>GSNLEERLRACMQKLACGKLTGISDPVTVKTSGSRFGSWMTDPLAPEGDNRVWYMDGYHNNRFVREYKSMVDFMNTDNFTSHRLPHPWSGTGQVVYNGSIYFNKFQSHIIIRFDLKTETILKTRSLDYAGYNNMYHYAWGGHSDIDLMVDENGLWAVYATNQNAGNIVISKLDPVSLQILQTWNTSYPKRSAGEAFIICGTLYVTNGYSGGTKVHYAYQTNASTYEYIDIPFQNKYSHISMLDYNPKDRALYAWNNGHQTLYNVTLFHAAAHHHHHH[2x]

Olfactomedin-1 (Olfm1; also known as Noelin or Pancortin) is a highly-expressed secreted brain and retina protein and its four isoforms have different roles in nervous system development and function. Structural studies showed that the long Olfm1 isoform BMZ forms a disulfide-linked tetramer with a V-shaped architecture. The tips of the Olfm1 “V” each consist of two C-terminal β-propeller domains that enclose a calcium binding site. The highly conserved monomeric Olf domain has a five-bladed β-propeller fold with a central metal ion binding site.

A dimeric variant containing part of the coiled coil and Olf domain, corresponding to our previously crystallised proteolysis fragment, was designed with domain boundaries 212–478 (UNIPROT numbering). This includes Cys221 that forms an inter-chain disulfide and covalently locks this construct in a dimeric form. We crystallised the dimeric form of Olfm1coil-Olf, after deglycosylation with Endo-H, with calcium chloride present in the buffer. The Olfm1coil-Olf structure reported previously was not deglycosylated indicating that the glycans did not contribute substantially to the crystal packing. The β-propellers in the Z isoforms are covalently dimerised by an inter-chain disulfide bond (formed by Cys221-Cys221) at the C-terminus of the preceding coiled-coil domain. Only about a third of this recombinant Olfm1coil-Olf sample formed disulfide-linked dimers as in the crystal structure, yet the monomeric and dimeric fractions could be separated from each other by two rounds of SEC (see Materials and methods section for details). The switch loop forms part of this top face in the calcium-bound state and alters the properties of this surface. In the calcium-bound state the top face still consists of conserved residues and is devoid of glycans. Another putative region of interaction is the crevice between the two Olf domains, flanked by β-propeller blades 4 and 5.> EEKKKKRSGFRDRKVMEYENRIRAYSTPDKIFRYFATLKVISEPGEAEVFMTPEDFVRSITPNEKQPEHLGLDQYIIKRFDGKKISQEREKFADEGSIFYTLGECGLISFSDYIFLTTVLSTPQRNFEIAFKMFDLNGDGEVDMEEFEQVQSIIRSQTSMGMRHRDRPTTGNTLKSGLCSALTTYFFGADLKGKLTIKNFLEFQRKLQHDVLKLEFERHDPVDGRITERQF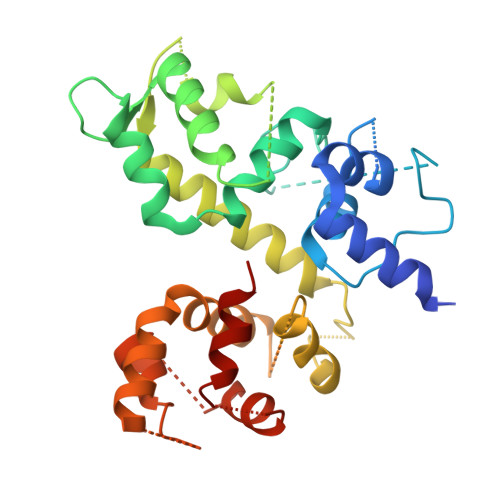GGMLLAYSGVQSKKLTAMQRQLKKHFKEGKGLTFQEVENFFTFLKNINDVDTALSFYHMAGASLDKVTMQQVARTVAKVELSDHVCDVVFALFDCDGNGELSNKEFVSIMKQRLMRG>YPTAIDVRDIPTTQLEDFKFWVQYAAATYCPNNYVAKDGEKLNCSVGNCPDVEAAGSTVKLSFSDDTITDTAGFVAVDNTNKAIVVAFRGSYSIRNWVTDATFPQTDPGLCDGCKAELGFWTAWKVVRD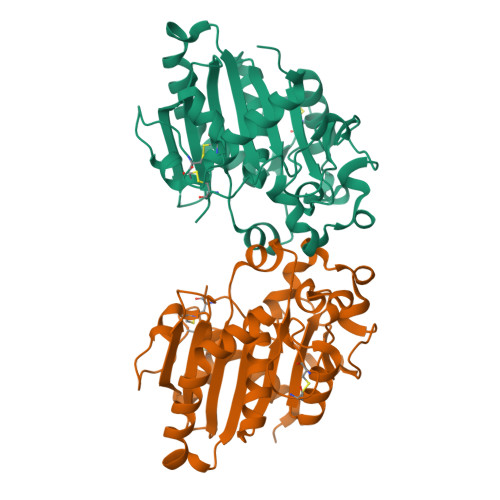RIIKTLDELKPEHSDYKIVVVGHSLGAAIASLAAADLRTKNYDAILYAYAAPRVANKPLAEFITNQGNNYRFTHNDDPVPKLPLLTMGYVHISPEYYITAPDNTTVTDNQVTVLDGYVNFKGNTGTSGGLPDLLAFHSHVWYFIHADACKGPGLPLR[2x]> MSQSNRELVVDFLSYKLSQKGYSWSQFSDVEENRTEAPEGTESEAVKQALREAGDEFELRYRRAFSDLTSQLHITPGTAYQSFEQVVNELFRDGVNWGRIVA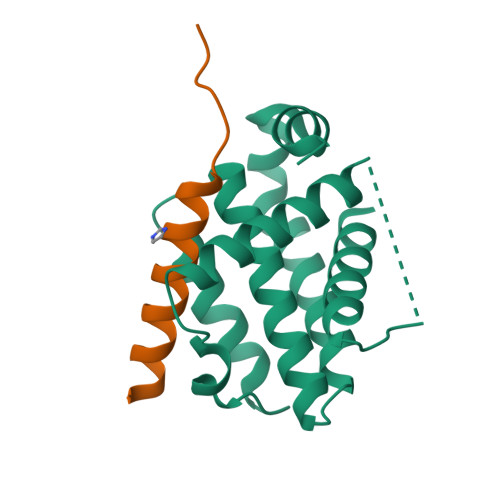FFSFGGALCVESVDKEMQVLVSRIAAWMATYLNDHLEPWIQENGGWDTFVELYGNNAAAESRKGQER;> SESQEDIIRNIARHLAQVGDSMDRSIPPGLVNGL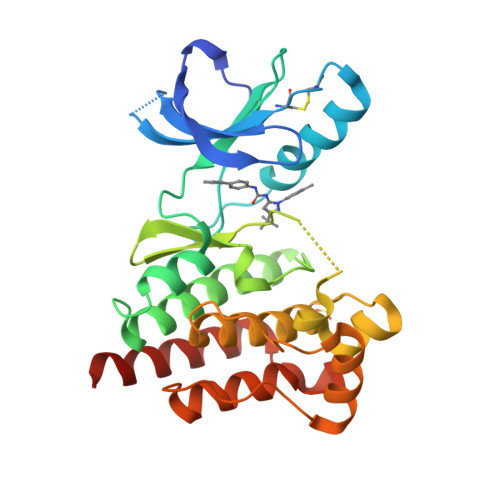>[2x]GSGSTRDYEIQRERIELGRCIGEGQFGDVHQGIYMSPENPALAVAIKTCKNCTSDSVREKFLQEALTMRQFDHPHIVKLIGVITENPVWIIMELCTLGELRSFLQVRKYSLDLASLILYAYQLSTALAYLESKRFVHRDIAARNVLVSSNDCVKLGDFGLSRYMEDSTYYKASKGKLPIKWMAPESINFRRFTSASDVWMFGVCMWEILMHGVKPFQGVKNNDVIGRIENGERLPMPPNCPPTLYSLMTKCWAYDPSRRPRFTELKAQLSTILEEEKAQQEE> MKKNG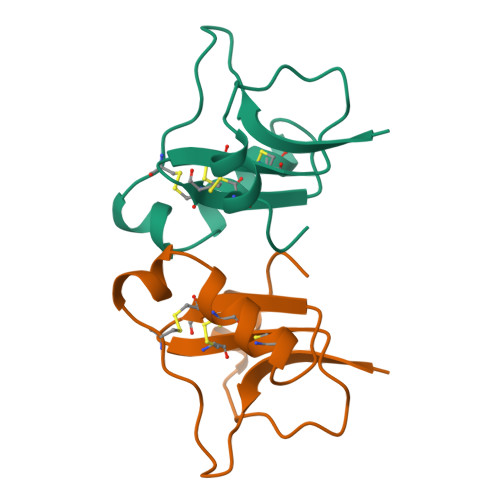YPLDRNGKTTECSGVNAIAPHYCNSECTKVYYAESGYCCWGACYCFGLEDDKPIGPMKDITKKYCDVQIIPS>[4x]ALH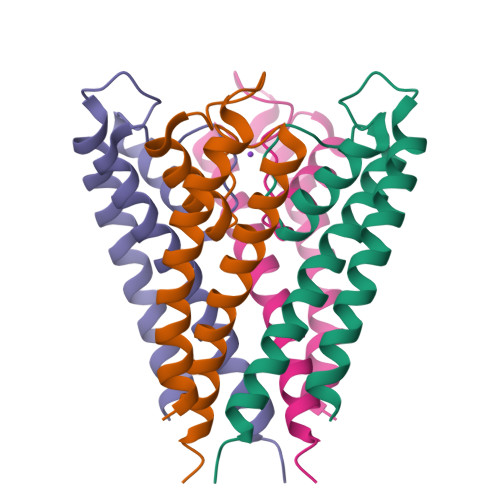WRAAGAATVLLVIVLLAGSYLAVLAERGAPGAQLITYPRALWWSVETATTVGYGDLYPVTLWGRCVAVVVMVAGITSFGLVTAALATWFVGREQ> MRAVRLVEIGKPLSLQEIGVPKPKGPQVLIKVEAAGVCHSDVHMRQGRFGNLRIVEDLGVKLPVTLGHEIAGKIEEVGDEVVGYSKGDLVAVNPWQGEGNCYYCRIGEEHLCDSPRWLGINFDGAYAEYVIVPHYKYMYKLRRLNAVEAAPLTCSGITTYRAVRKASLDPTKTLLVVGAGGGLGTMAVQIAKAVSGATIIGVDVREEAVEAAKRAGADYVINASMQDPLAEIRRITESKGVDAVIDLNYSEKTLSVYPKALAKQGKYVMVGLFGADLHYHAPLI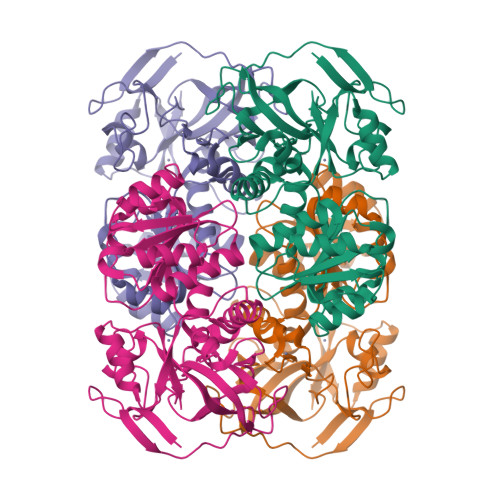TLSEIQFVGSLVGNQSDFLGIMRLAEAGKVKPMITKTMKLEEANEAIDNLENFKAIGRQVLIP> TARXSTGG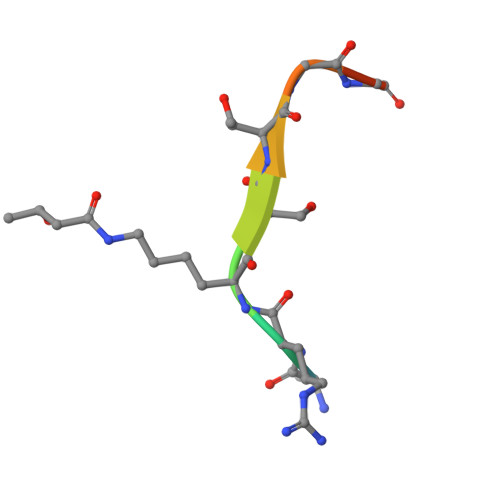KA>[2x]MGVTKTPLYETLNESSAVALAVKLGLFPSKSTLTCQEIGDGNLNYVFHIYDQEHDRALIIKQAVPYAKVVGESWPLTIDRARIESSALIRQGEHVPHLVPRVFYSDTEMAVTVMEDLSHLKIARKGLIEGENYPHLSQHIGEFLGKTLFYSSDYALEPKVKKQLVKQFTNPELCDITERLVFTDPFFDHDTNDFEEELRPFVEKLWNNDSVKIEAAKLKKSFLTSAETLIHGDLHTGSIFASEHETK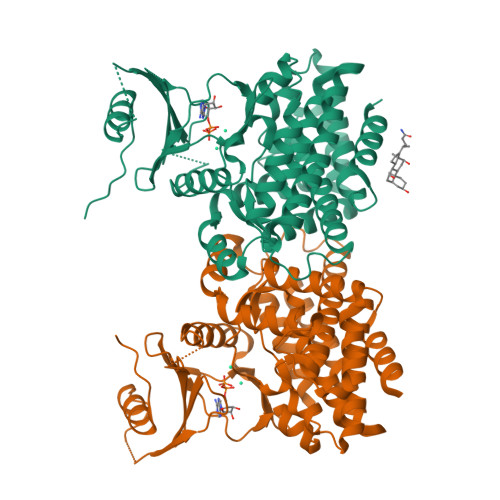VIDPEFAFYGPIGFDVGQFIANLFLNALSRDGADREPLYEHVNQVWETFEETFSEAWQKDSLDVYANIDGYLTDTLSHIFEEAIGFAGCELIRRTIGLAHVADLDTIVPFDKRIGRKRLALETGTAFIEKRSEFKTITDVIELFKLLVKE>MKHHHHHHHHHHSAGLEVLFQGPYVQAFDSLLANPVAEYLKMSKEIGGDVQKHAEMVHTGLKLERALLATASQCQQPAGNKLSDLLAPISEQIQEVITFREKNRGSKFFNHLSAVSESIQALGWVALAAKPGPFVKEMNDAAMFYTNRVLKEYRDVDKKHVDWVRAYLSIWTELQAYIKEFHTTGLAWSKTGPVAKEL[4x]

Another actin-binding protein implicated in filament disassembly is cyclase-associated protein (CAP). It is conserved in evolution from protozoan parasites through yeasts and plants to animals, and is thus among the small number (<10) of core actin-binding proteins present in all eukaryotes. CAP is a relatively large multidomain protein, which can self-assemble into oligomers, most likely hexamers. Here, we reveal that CAP promotes rapid actin filament disassembly by accelerating pointed end depolymerization of cofilin-decorated actin filaments.

The N-terminal HFD domain of CAP is critical for actin filament disassembly in vitro and in cells. Interestingly, the dimeric HFD domain was able to strongly accelerate actin filament depolymerization at much lower concentration when compared to the monomeric HFD domain. These data demonstrate that the HFD domain is the functionally minimal unit for actin filament pointed end depolymerization, and that its oligomerization decreases the effective protein concentration needed for this activity.> ALPQTVRIGTATTYAPFSSKDAKGEFIGFDIDLGNEMCKRMQVKCTWVASDFDALIPSLKAKKIDAIISSLSIT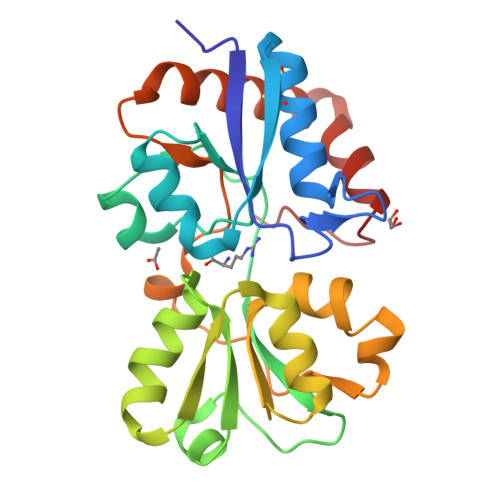DKRQQEIAFSDKLYAADSRLIAAKGSPIQPTLESLKGKHVGVLQGSTQEAYANDNWRTKGVDVVAYANQDLIYSDLTAGRLDAALQDEVAASEGFLKQPAGKEYAFAGPSVKDKKYFGDGTGVGLRKDDTELKAAFDKALTELRQDGTYDKMAKKYFDFNVYGD>FKRIVQ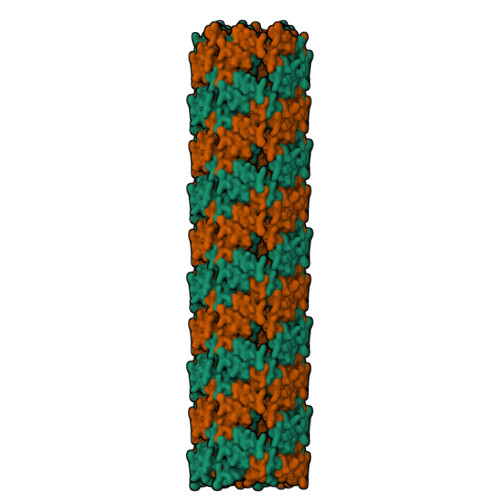RIKDFLR[2x]> MNTPEHMTAVVQRYVAALNAGDLDGIVALFADDATVEDAVGSEPRSGTAAIREFYANSLKLPLAVELTQEVRAVANEAAFAFIVSFEYQGRKTVVAPIDHFRFNGAGKVVSMRALFGE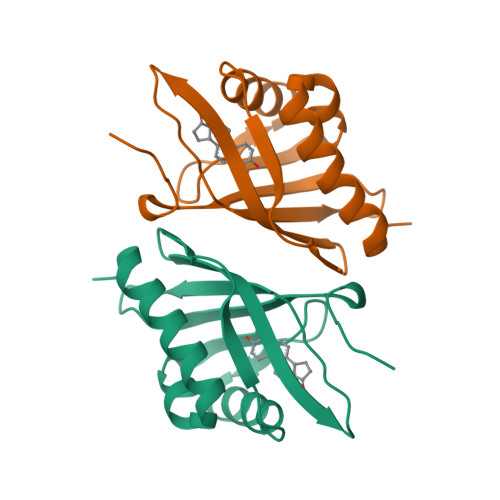KNIHAGA> VVGGLVALRGAHPYIAALYWGHSFCAGSLIAPCWVLTAAHCLQDRPAPEDLTVVLGQERRNHSCEPCQTLAVRSYRLHEAFSPVSYQHDLALLRLQEDADGSCALLSPYVQPVSLPSGAARPSETTLCQVAGWGHQFEGAEEYASFLQEAQVPFLSLERCSAPDVHGSSILPGMLCAGFLEGGTDACQGDSGGPLVCEDQAAERRLTLQGIISWGSGCGDRNKPGVYTDVAYYLAWIREHTVSHHTGTRHHHHHH

FXII circulates in the blood as an 80-kDa single-chain polypeptide zymogen with no detectable enzymatic activity. The FXII Arg353–Val354 peptide bond is cleaved by kallikrein, generating α-FXIIa, which has a heavy chain of 50 kDa, connected to a light chain of 28 kDa by the Cys340–Cys467 disulfide bridge. Subsequent cleavage of α-FXIIa results in loss of the heavy chain and generation of the isolated protease domain termed β-FXIIa, which contains only a nine amino acid peptide heavy chain remnant disulfide bonded to the protease domain. Here, we describe the first crystal structures of the FXII protease domain, which reveals a zymogen-like conformation.

The recombinant proteins investigated were FXIIac, which has the native N-terminus, and a zymogen-like protease FXIIc, in which the N-terminus is blocked by the presence of two additional amino acids, Arg and Ser. Using the recombinant FXIIac protease in crystallization experiments, we followed a similar approach as the FXI protease (FXIac) of cocrystallization with the inhibitors PCK, PPACK, and corn trypsin inhibitor. FXIIac crystallized both in the presence and in the absence of PPACK at 10 °C, and the FXIIac crystal structure was determined by molecular replacement with the structure of the homologous HGFA protease and refined to an R-factor of 0.219 (data collection and refinement statistics are summarized in Table 1). A key feature that identifies the FXIIac structure as a zymogen is the absence of an oxyanion hole (Gly193 and Ser195) and a buried zymogen-like conformation of the Asp194 side chain, whereby it forms hydrogen bonds with the main chain nitrogen of Trp141. A second feature is that residues 182–183 from the 180-loop and residues 217–221 from the 220-loop of the S1 pocket are not visible in the electron density. In one crystal form, the S1 pocket loops are partially flexible, which is typical of a zymogen. The N-terminus is not observed in the FXIIac electron density, and Val16–Leu23 are presumed to be flexible, and do not efficiently insert into the core of the protease domain in this context (see discussion). We have previously observed in the FXI zymogen crystal structure, where there are no crystal packing contacts in the area of the active site, that the 180-loop and 220-loop are also not present in the electron density, suggesting S1 loop flexibility. The FXIIac zymogen conformation was unexpected, but is in agreement with the enzyme kinetic data described above, which showed that FXIIac has reduced catalytic activity as compared with β-FXIIa. The zymogen conformation of FXIIac is unexpected, as protease constructs for u-Pa, FXIa and trypsin lacking a heavy chain remnant have been crystallized in the active conformation.>MGSSHHHHHHSSGENLYFQGHMHESRLASARLYLCTDARRERGDLAQFAEAALAGGVDIIQLRDKGSPGEL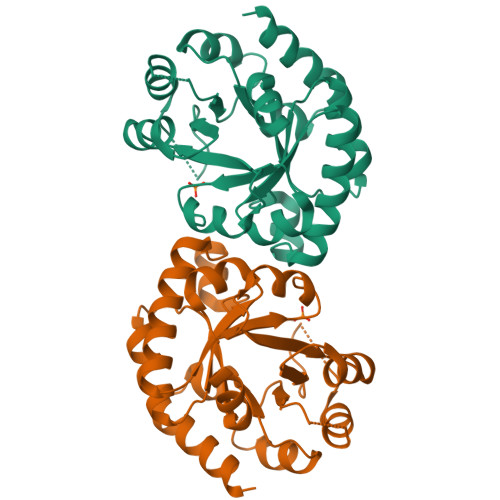RFGPLQARDELAACEILADAAHRYGALFAVNDRADIARAAGADVLHLGQRDLPVNVARQILAPDTLIGRSTHDPDQVAAAAAGDADYFCVGPCWPTPTKPGRAAPGLGLVRVAAELGGDDKPWFAIGGINAQRLPAVLDAGARRIVVVRAITSADDPRAAAEQLRSALTAAN[2x]>[15x]MNNLYRELAPVTDAAWHEIETEAIRTFKRHIAGRRVVDVSEPSGPVTAAVSTGHLRDISPPGDGVVAHLRESKPLVRLRVPFTVTRSAIDDVERGSQDSDWDPVKAAAKKLAFVEDRAIFEGYPAAQIDGIRQCTSNPVLQLPDDARDITDVIAQALSELRLAGVDGPYSVLLSAEVYTKVSETTEHGYPIREHLNRLVDGDIIWAPAIDGAFVLSTRGGDFDLRLGTDVSIGYLS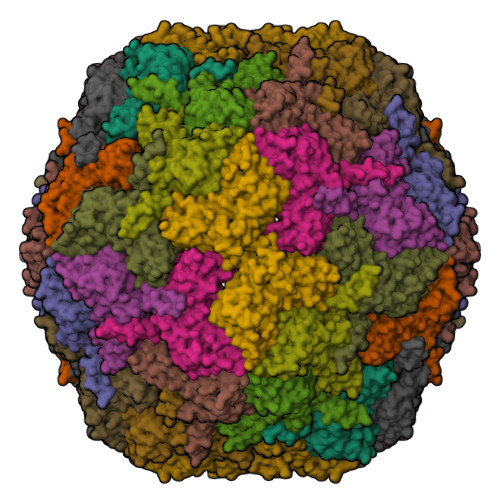HDAETVQLYLEETLTFLCYTSEASVALTP> MNFDYIAHARQDSSKNWHSHPLQKHLQKVAQLAKRFAGRYGSLFAEYAGLLHDLGKFQESFQKYIRNASGFEKENAHLEDVESTKLRKIPHSTAGAKYAVERLNPFFGHLLAYLIAGHHAGLADWYDKGSLKRRLQQADDELAASLSGFVESSLPEDFFPLSDDDLMRDFFAFWEDGAKLEELHIWMRFLFSCLVDADFLDTEAFMNGYADADTAQAAGLRPKFPGLDELHRRYEQYMAQLSEKADKNSSLNQERHAILQQCFSAAETDRTLFSLTVPTGGGKTLASLGFALKHALKFGKKRIIYAIPFTSIIEQNANVFRNALGDDVVLEHHSNLEVKEDKETAKTRLATENWDAPLIVTTNVQLFESLFAAKTSRCRKIHNIADSVVILDEAQQLPRDFQKPITDMMRVLARDYGVTFVLCTATQPELGKNIDAFGRTILEGLPDVREIVADKIALSEKLRRVRIKMPPPNGETQSWQKIADEIAARPCVLAVVNTRKHAQKLFAALPSNGIKLHLSANMCATHCSEVIALVRRYLALYRAGSLHKPLWLVSTQLIEAGVDLDFPCVYRAMAGLDSIAQAAGRCNREGKLPQLGEVVVFRAEEGAPSGSLKQGQDITEEMLKAGLLDDPLSPLAFAEYFRRFNGKGDVDKHGITTLLTAEASNENPLAIKFRTAAERFHLIDNQGVALIVPFIPLAHWEKDGSPQIVEANELDDFFRRHLDGVEVSEWQDILDKQRFPQPPDNSFGQTDQPLLPEPFESWFGLLESDPLKHKWVYRKLQRYTITVYEHELKKLPEHAVFSRAGLLVLDKGYYKAVLGADFDDAAWLPENSVLGGSVGPKKKRKVLEHHHHHH

Among many types of CRISPR-Cas systems, Type I CRISPR-Cas systems are most abundant, with target interference depending on a multi-subunit, RNA-guided complex known as Cascade that recruits a transacting helicase nuclease, Cas3, to degrade the target. Cas3 is a multi-domain protein consisting of approximately 800–900 amino acids in the Type I CRISPR–Cas system and is responsible for the actual cleavage of target DNA. Our structural study revealed that, like other types of Cas3, NlaCas3 is distinctly composed of three major domains including the HD nuclease domain, RecA-like helicase domain, and CTD.

In the present study, we elucidated the first structure of standalone Type I-C Cas3 from Neisseria lactamica (NlaCas3). Following purification, the target protein was successfully crystallized, and its crystal structure was determined at a resolution of 2.17 Å using the molecular replacement (MR) phasing method. The crystal was categorized under the space group C2, with a single molecule present in the asymmetric unit. The overall tertiary structure of NlaCas3 exhibited a typical structural fold of Cas3, compactly arranged with the N-terminal histidine–aspartate (HD) nuclease domain and RecA-like helicase domains positioned adjacent to each other, thereby forming a functional unit that is capable of DNA cleavage and unwinding. Two prominent round-shaped electron densities, characteristic of metal-ion density, were observed around the active site of HD nuclease of NlaCas3. This metal ion density was coordinated by O and N atoms from the side chains of residues H8, H25, H52, D53, H118 and H119. Additionally, ICP–MS results indicating a 2:1 ratio of Fe2+ to Mn2+ binding indicated that the metal ions in the active site of HD nuclease domain corresponded to two Fe2+ ions. Conversely, in our isolated NlaCas3 structure, Fe2+ ions, which inhibit NlaCas3 activity, were detected, indicating an inactive form. When comparing our standalone NlaCas3 structure in its presumed inactive form to the structure of Cas3 bound to the actual substrate DNA within the Cascade complex, we observed that the HD gate loop from the HD nuclease domain and RecA1 gate loop from the RecA1 domain in our NlaCas3 structure blocked the active site of HD nuclease. When we compared our standalone NlaCas3 structure with that of NlaCas3 in complex with Cascade, the anchor loop of NlaCas3, which is utilized for binding with Cas8 in the complex, underwent significant structural changes when NlaCas3 was present alone and positioned in a completely opposite direction.> GKKDTQSITLEELAKIIKKCKHVVALTGSGTSAESNIPSFRGSSN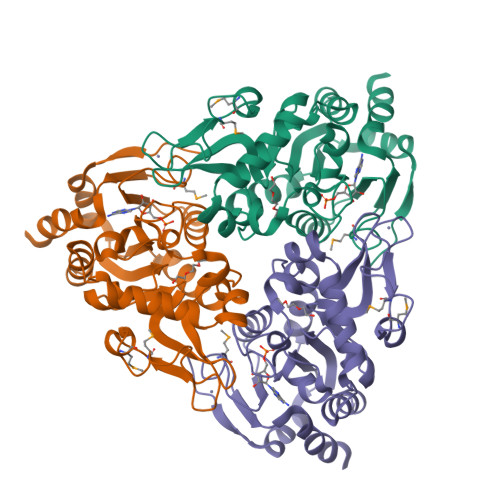SIWSKYDPRIYGTIWGFWKYPEKIWEVIRDISSDYEIEINNGHVALSTLESLGYLKSVVTQNVDGLHEASGNTKVISLHGNVFEAVCCTCNKIVKLNKIMLQKTSHFMHQLPPECPCGGIFKPNIILFGEVVSSDLLKEAEEEIAKCDLLLVIGTSSTVSTATNLCHFACKKKKKIVEINISKTYITNKMSDYHVCAKFSELTKVANILKGSSEKNKKIM>[2x]MHHHHHHMLENKLGIINQLELNRVEERVSKENAKRLYDSGDIDRIEVGTFKGLSYIHNYLFEDIYEFAGKVRSQNISKGNFRFAPVMYLEIALEHIDKMPQRNLDEIVAKYVEMNIAAPFREGNGRATRIWLDLILKKELKRVVDWNLINKEDYLSAMERSPVKDLEIKYLISNALTDKINDREIFMKGIDISYYYEGYTEYNVDEL

The most frequent PTM reaction catalyzed by FIC enzymes is the addition of AMP using ATP as a cofactor, coined AMPylation or adenylylation. Enterococcus faecalis FIC belongs to class III FIC proteins, which are comprised of a single FIC domain and carry an autoinhibitory glutamate in their C-terminal α-helix. We discover that EfFIC has both AMPylation and deAMPylation activities borne by the same active site. Furthermore, the conserved glutamate implements a Ca2+-controlled metal switch that tunes the balance between these activities without conformational change.

We determined crystal structures of unbound, phosphate-bound, AMP-bound, and ATPγS-bound wild-type EfFIC (EfFICWT) and of unbound and sulfate-bound EfFIC carrying a mutation of the catalytic histidine into an alanine (EfFICH111A). All EfFIC monomers resemble closely to each other and to structures of other class III FIC proteins. Mutation of the catalytic histidine (H111A), of the metal-binding acidic residue in the FIC motif (E115A), or of the inhibitory glutamate completely impaired deAMPylation of AMP-FAMEfFICE190G (mutant panels).Contractile bacteriophages of the family Myoviridae (i.e. T4), R-type pyocins and the type VI secretion system (T6SS) of Gram-negative bacteria are evolutionarily related nano-scale injection machines that puncture target cell membranes using a shared contraction mechanism. TssA subunits are enigmatic as they possess a conserved N-terminal region of unknown function, previously identified as ImpA_N (PFAM: PF0681226), whereas sequences located C-terminal to this region are highly divergent. Consistent with this, phylogenetic analysis has suggested that the TssA family can be subdivided into three clades (TssA1, TssA2 and TssA3). The structural studies presented here show that TssA1B, TssA2A and TssA2B possess structurally diverse CTDs that lead to distinct overall architectures for their respective complexes.

We also provide the structure of an Nt2-CTD TssA2A construct, demonstrating that 10 subunits assemble into a complex with distinct five-fold symmetry rather than the six-fold symmetry seen in EAEC TssA2B. The structure of crystals of an Ah His6.TssA2A Nt2-CTD construct (R232-K478) was successfully determined to 3.13 Å through molecular replacement using the coordinates of the Ah TssA2A Nt2 dimer as a search model. This identified the position of five dimers of the TssA2A Nt2 domain (R232 to L374, helices α1–α7) in the asymmetric unit, which did not appear to be arranged with any obvious symmetry with respect to each other. The remaining C-terminal residues of each of the 10 subunits (chains A-J) were organised into a separate domain (the CTD) consisting of five α-helices (G388-L472, α8–α12). In the assembled TssA2A CTD decamer two distinct two-fold interfaces can be identified. In the first, a two-fold related interface (shown by PISA32 to be 530 Å2) is formed primarily through interactions between residues from the extended loop linking α11 and α12 and the N-terminal end of α10 and their symmetry-related partners. In the second, more extensive interface (950 Å2), the WEP-mediated dimers assemble around the five-fold axis through interactions between the surface of helices α9, α10 and α11 and their two-fold related symmetry mates to form a mixed interface of hydrophobic/hydrophilic contacts. However, restrictions imposed by the maximum length of the absent linker residues and the relative orientations of the Nt2 and CTD domains allowed the unambiguous assignment of the Nt2 domains to their corresponding CTD (i.e. in the same polypeptide chain). This revealed that in the decameric Ah TssA2A Nt2-CTD complex, the Nt2 domains are not related by the five-fold symmetry exhibited by their corresponding CTDs. Moreover, as a result of the flexible linker, the Nt2 dimers have quite different orientations with respect to the five-fold axis, with angular rotations of up to ~60° about the vertical axis, and ~45° and ~60° about the horizontal and torsional axes, respectively.

>MGSSHHHHHHSGAPGVDVDSSNDRAWRQTQLKVAELLIERQPEVAVGYRLRRHAVWAGITAVPMSGAGNKTPLAPMSADMVDEYRAAMNAPDQGLWQRIEQSLTLAPYWFEGHRLSAEVAEKLGFGAVAQAIAEELGTFLQRLPALRELAFSDGSPFLSPECSRWLQPAKGGSAGIGEAGLAEEVAQRHGEQGIAAALALLDERIAQLKEPRDRFHALLVQAELLAQEGMEALARQHYQHLWQEASRLGLSHWEPGLVNRLESLAAPLSK[10x]> MASQSQGIQQ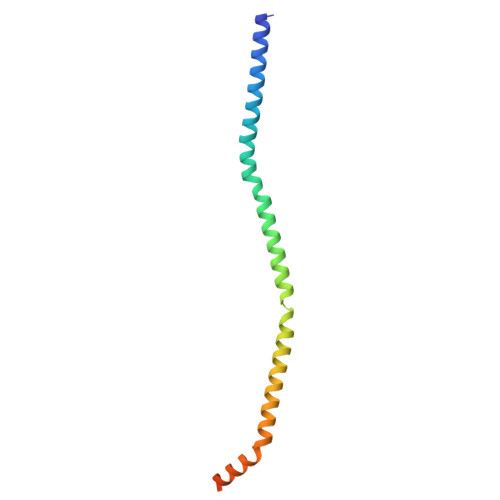LLQAEKRAAEKVADARKRKARRLKQAKEEAQMEVEQYRREREQEFQSKQQAAMGSQGNLSAEVEQATRRQVQGMQSSQQRNRERVLTQLLGMVCDVRPQVHPNYRITV> RKTITGVFNSFDSLTWTRSVEYVYKGPETPTWNAVLGWSLNSTTADPGDTFTLILPCVFKFITTQTSVDLTADGVSYATCDFNAGEEFTTFSSLSCTVNSVSVSYARVSGTVKLPITFNVGGTGSSVDLADSKCFTAGKNTVTFMDGDTKISTTVDFDASPVSPSGYITSSRIIPSLNKLSSLFVVPQCENGYTSGIMG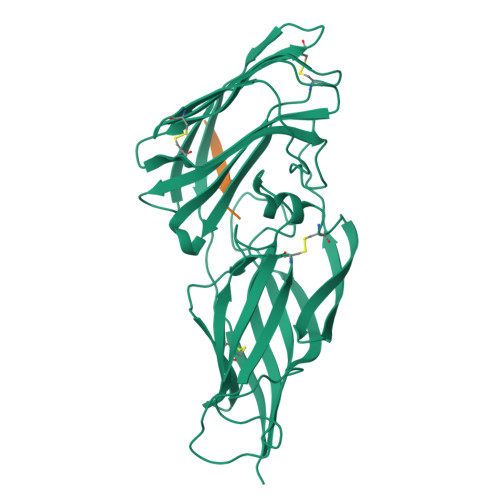FVASNGATIDCSNVNIGISKGLNDWNFPVSSESFSYTKTCTSTSITVEFQNVPAGYRPFVDAYISAENIDKYTLTYANEYTCENGNTVVDPFTLTWWGYKNSEADSDGDVIVV;> GEGQQHHLGGAKQAGDV One extracellular protein family that arose through domain replication and gene duplication is the gel-forming mucins, huge glycoproteins that coat and protect the epithelia in the lungs, intestines, and other organs. A remarkable variation on the theme of mucins arose with the evolution of the complex vasculature in the vertebrate lineage. von Willebrand factor (VWF), a glycoprotein responsible for hemostasis, has a similar domain organization and is homologous to mucins in its amino- and carboxyl-terminal regions. Under acidic conditions, the amino termini of mucins and VWF form noncovalent intermolecular interactions that juxtapose VWD3 assemblies from different CTCK-linked dimers. We present residue-resolution structures of VWF and MUC2 amino-terminal segment tubules, enabling comparison between them and an analysis of the features that stabilize each one.

Due to furin cleavage during recombinant protein production, we assembled the VWF tubules from the D3 dimer and D1D2 fragments purified separately. The VWF and MUC2 tubules also both display twofold symmetry perpendicular to the helix axis. They differ, however, in that the VWF tubule is a one-start helix, whereas the MUC2 tubule is a two-start helix. The VWF tubule has a helical twist of 86.0° (about 4.2 subunits per turn) and an axial rise of 2.85 nm per subunit. The VWF subregion map contained two adjacent beads along the path of the helix at an overall nominal resolution of 3.4 Å, and both beads were of similar resolution. Aside from the furin cleavage region, the remainder of the VWF bridge is highly ordered. The E2 module of a VWF protein molecule arising from one bead makes numerous contacts with the D1 and D2 assemblies from different protein molecules in the neighboring bead. This ternary interaction may stabilize both the bead assembly and the relative orientation of beads. The contact between the bridge and D1 includes a cation–π interaction between Y730 and R202, while the contact between the bridge and D2 includes cation–π interactions between F716 and H460 and between F722 and R442. In the same region, a row of salt bridges is made by the intercalation of residues E714 and D724 from the bridge between R442 and K459 in D2, and another salt bridge was found between Asp720 and Arg505. Further supporting the interaction between beads in VWF, direct D2–D2 contacts are made at the interface between beads (Left).

>[4x]MIPARFAGVLLALALILPGTLCAEGTRGRSSTARCSLFGSDFVNTFDGSMYSFAGYCSYLLAGGCQKRSFSIIGDFQNGKRVSLSVYLGEFFDIHLFVNGTVTQGDQRVSMPYASKGLYLETEAGYYKLSGEAYGFVARIDGSGNFQVLLSDRYFNKTCGLCGNFNIFAEDDFMTQEGTLTSDPYDFANSWALSSGEQWCERASPPSSSCNISSGEMQKGLWEQCQLLKSTSVFARCHPLVDPEPFVALCEKTLCECAGGLECACPALLEYARTCAQEGMVLYGWTDHSACSPVCPAGMEYRQCVSPCARTCQSLHINEMCQERCVDGCSCPEGQLLDEGLCVESTECPCVHSGKRYPPGTSLSRDCNTCICRNSQWICSNEECPGECLVTGQSHFKSFDNRYFTFSGICQYLLARDCQDHSFSIVIETVQCADDRDAVCTRSVTVRLPGLHNSLVKLKHGAGVAMDGQDVQLPLLKGDLRIQHTVTASVRLSYGEDLQMDWDGRGRLLVKLSPVYAGKTCGLCGNYNGNQGDDFLTPSGLAEPRVEDFGNAWKLHGDCQDLQKQHSDPCALNPRMTRFSEEACAVLTSPTFEACHRAVSPLPYLRNCRYDVCSCSDGRECLCGALASYAAACAGRGVRVAWREPGRCELNCPKGQVYLQCGTPCNLTCRSLSYPDEECNEACLEGCFCPPGLYMDERGDCVPKAQCPCYYDGEIFQPEDIFSDHHTMCYCEDGFMHCTMSGVPGSLLPDAVLSSPLSHRSKRSLSCRPPMVKLVCPADNLRAEGLECTKTCQNYDLECMSMGCVSGCLCPPGMVRHENRCVALERCPCFHQGKEYAPGETVKIGCNTCVCRDRKWNCTDHVCDATCSTIGMAHYLTFDGLKYLFPGECQYVLVQDYCGSNPGTFRILVGNKGCSHPSVKCKKRVTILVEGGEIELFDGEVNVKRPMKDETHFEVVESGRYIILLLGKALSVVWDRHLSISVVLKQTYQEKVCGLCGNFDGIQNNDLTSSNLQVEEDPVDFGNSWKVSSQCADTRKVPLDSSPATCHNNIMKQTMVDSSCRILTSDVFQDCNKLVDPEPYLDVCIYDTCSCESIGDCACFCDTIAAYAHVCAQHGKVVTWRTATLCPQSCEERNLRENGYECEWRYNSCAPACQVTCQHPEPLACPVQCVEGCHAHCPPGKILDELLQTCVDPEDCPVCEVAGRRFASGKKVTLNPSDPEHCQICHCDVVNLTCEACQEPG L-arginine oxidase (AROD, EC 1.4.3.25) is an oxidoreductase that catalyses the deamination of L-arginine, with flavin adenine dinucleotide (FAD) as a cofactor. Recently identified AROD from Pseudomonas sp. TPU 7192 (PT-AROD) demonstrates high selectivity for L-arginine. This enzyme is useful for accurate assays of L-arginine in biological samples.

Comparative analysis of this structure with that determined using X-ray crystallography reveals open and closed forms of the lid-like loop at the entrance to the substrate pocket.

>[4x]MHHHHHHMSQTQPLDVAIIGGGVSGTYSAWRLQEAQGDHQRIQLFEYSDRIGGRLFSINLPGLPNVVAEVGGMRWMPATKDNTGGHVMVDKLVGELKLESKNFPMGSNLPDKDPVGAKDNLFYLRGERFRLRDFTEAPDKIPYKLAWSERGYGPEDLQVKVMHNIYPGFDKLSLAEQMQVKVFGKEIWRYGFWDLLYRVLSNEGYQFMKDAGGYEANVANASAVTQLPATEYSDKTVFLTLKKGFQALPLTLAKRFAEVPGGLIAGEQRIRMNRRLASVQFSDDTEYPYRLHFQATRTVDGKTSDVPGAEEIIHARQVILALPRRSLELIQSPLFDDPWLKENIDSVLVQSAFKLFLAYEQPWWRSQGLVAGRSVTDLPIRQCYYMGTECEQDGGEKTLNSLLMASYNDIGTVPFWKGLEDGAPFEGYQPKSLQGRIDANEVVPKMQYQISEEMVRIAQRQVTSLHDQIELPAPYSAVYHAWDADPFGGGWHEWKANYRLDLIIQRMRHPVQEQEVYIVGEAYSYGQGWVEGALTTAESTLQDFFGLPRPAWLPEAYQLLPAPAPVDIDNPPALACTDCKKTLTEVTEFAYTGIKA>SLPHQPIPPSLGEKDLSDPFNFLFSSNKITLRKLYDLTKNVDFDQLRQNECKKNITLSKFWEKSEQRNVPEDDNWERFYSNIGSCSVYSDDQMIDNLLHDLNTSPIKHVHIMDGGTQVKFVFTFKNDKQAVFKPMRFGRDYESDPNHFYFSDFERHHAEIATFHLDRVLGFRRAIPTVGRVLNMTTELFEKAEKKL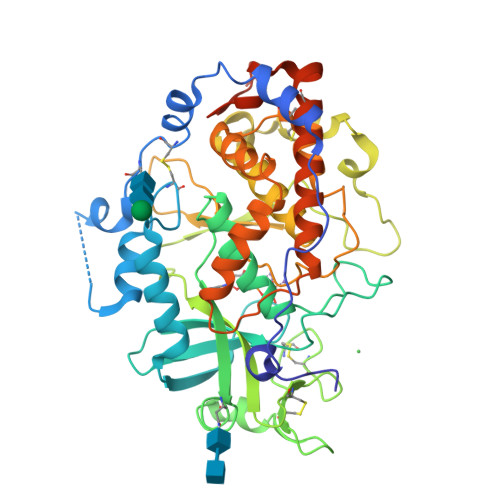KKTFFFSPAKNFCFVSRCDYYCDTTHAICGLPDMKEGSVQVFLPDESAVPRKHNRSPYRRTYSKKNQVAEWQSSMNYCTDKVKTKRQYAHGRRLLDLVDIHILDYLIGNQDRHHFESFNVFNDLPSYAIHLDHGRAFGRSDFDDDDIILPLRQCCILRPSTFQTLMNFYSTPKSLTKALHESLSKDPAHPILAYKHYPAMERRLAKIMSHILECFESRGVAEVLVAEYNNPDVSDAEQNDEEQSEEHQDKKDDKKTV[2x]> GEFAQECQNL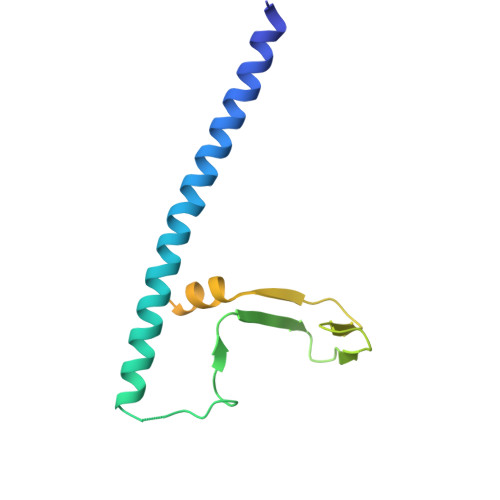EVERQRRLERIKQKQSQLQELILQQIAFKNLVQRNRHAEQQASRPPPPNSVIHLPFIIVNTSKKTVIDCSISNDKFEYLFNFDNTFEIHDDIEVLKRMGMACGLESGSCSAEDLKMARSLVPKALEPYVTEMAQGTVGGVFITTA>MSRIEKMSILGVRSFGIEDKDKQIITFFSPLTILVGPNGAGKTTIIECLKYICTGDFPPGTKGNTFVHDPKVAQETDVRAQIRLQFRDVNGELIAVQRSMVCTQKSKKTEFKTLEGVITRTKHGEKVSLSSKCAEIDREMISSLGVSKAVLNNVIFCHQEDSNWPLSEGKALKQKFDEIFSATRYIKALETLRQVRQTQGQKVKEYQMELKYLKQYKEKACEIRDQITSKEAQLTSSKEIVKSYENELDPLKNRLKEIEHNLSKIMKLDNEIKALDSRKKQMEKDNSELEEKMEKVFQGTDEQLNDLYHNHQRTVREKERKLVDCHRELEKLNKESRLLNQEKSELLVEQGRLQLQADRHQEHIRARDSLIQSLATQLELDGFERGPFSERQIKNFHKLVRERQEGEAKTANQLMNDFAEKETLKQKQIDEIRDKKTGLGRIIELKSEILSKKQNELKNVKYELQQLEGSSDRILELDQELIKAERELSKAEKNSNVETLKMEVISLQNEKADLDRTLRKLDQEMEQLNHHTTTRTQMEMLTKDKADKDEQIRKIKSRHSDELTSLLGYFPNKKQLEDWLHSKSKEINQTRDRLAKLNKELASSEQNKNHINNELKRKEEQLSSYEDKLFDVCGSQDFESDLDRLKEEIEKSSKQRAMLAGATAVYSQFITQLTDENQSCCPVCQRVFQTEAELQEVISDLQSKLRLAPDKLKSTESELKKKEKRRDEMLGLVPMRQSIIDLKEKEIPELRNKLQNVNRDIQRLKNDIEEQETLLGTIMPEEESAKVCLTDVTIMERFQMELKDVERKIAQQAAKLQGIDLDRTVQQVNQEKQEKQHKLDTVSSKIELNRKLIQDQQEQIQHLKSTTNELKSEKLQISTNLQRRQQLEEQTVELSTEVQSLYREIKDAKEQVSPLETTLEKFQQEKEELINKKNTSNKIAQDKLNDIKEKVKNIHGYMKDIENYIQDGKDDYKKQKETELNKVIAQLSECEKHKEKINEDMRLMRQDIDTQKIQERWLQDNLTLRKRNEELKEVEEERKQHLKEMGQMQVLQMKSEHQKLEENIDNIKRNHNLALGRQKGYEEEIIHFKKELREPQFRDAEEKYREMMIVMRTTELVNKDLDIYYKTLDQAIMKFHSMKMEEINKIIRDLWRSTYRGQDIEYIEIRSDADENVSASDKRRNYNYRVVMLKGDTALDMRGRCSAGQKVLASLIIRLALAETFCLNCGIIALDEPTTNLDRENIESLAHALVEIIKSRSQQRNFQLLVITHDEDFVELLGRSEYVEKFYRIKKNIDQCSEIVKCSVSSLGFNVH[2x];>MSTADALDDENTFKILVATDIHLGFMEKDAVRGNDTFVTLDEILRLAQENEVDFILLGGDLFHENKPSRKTLHTCLELLRKYCMGDRPVQFEILSDQSVNFGFSKFPWVNYQDGNLNISIPVFSIHGNNDDPTGADALCALDILSCAGFVNHFGRSMSVEKIDISPVLLQKGSTKIALYGLGSIPDERLYRMFVNKKVTMLRPKEDENSWFNLFVIHQNRSKHGSTNFIPEQFLDDFIDLVIWGHEHECKIAPTKNEQQLFYISQPGSSVVTSLSPGEAVKKHVGLLRIKGRKMNMHKIPLHTVRQFFMEDIVLANHPDIFNPDNPKVTQAIQSFCLEKIEEMLENAERERLGNSHQPEKPLVRLRVDYSGGFEPFSVLRFSQKFVDRVANPKDIIHFFRHREQKEKTGEEINFGKLITKPSEGTTLRVEDLVKQYFQTAEKNVQLSLLTERGMGEAVQEFVDKEEKDAIEELVKYQLEKTQRFLKERHIDALEDKIDEEVRRFRETRQKNTNEEDDEVREAMTRARALRSQSEESASAFSADDLMSIDLAEQMANDSDDSISAATNKGRGRGRGRRGGRGQNSASRGGSQRGRADTGLETSTRSRNSKTAVSASRNMSIIDAFKSTRQQPSRNVTTKNYSEVIEVDESDVEEDIFPTTSKTDQRWSSTSSSKIMSQSQVSKGVDFESSEDDDDDPFMNTSSLRRNRRSGGSLEVLFQGPDYKDDDDKGTDYKDDDDK[2x];> MWKLLPAAGPAGGEPYRLLTGVEYVVGRKNCAILIENDQSISRNHAVLTANFSVTNLSQTDEIPVLTLKDNSKYGTFVNEEKMQNGFSRTLKSGDGITFGVFGSKFRIEYEPLVACSSCLDVSGKTALNQAILQLGGFTVNNWTEECTHLVMVSVKVTIKTICALICGRPIVKPEYFTEFLKAVESKKQPPQIESFYPPLDEPSIGSKNVDLSGRQERKQIFKGKTFIFLNAKQHKKLSSAVVFGGGEARLITEENEEEHNFFLAPGTCVVDTGITNSQTLIPDCQKKWIQSIMDMLQRQGLRPIPEAEIGLAVIFMTTKNYCDPQGHPSTGLKTTTPGPSLSQGVSVDEKLMPSAPVNTTTYVADTESEQADTWDLSERPKEIKVSKMEQKFRMLSQDAPTVKESCKTSSNNNSMVSNTLAKMRIPNYQLSPTKLPSINKSKDRASQQQQTNSIRNYFQPSTKKRERDEENQEMSSCKSARIETSCSLLEQTQPATPSLWKNKEQHLSENEPVDTNSDNNLFTDTDLKSIVKNSASKSHAAEKLRSNKKREMDDVAIEDEVLEQLFKDTKPELEIDVKVQKQEEDVNVRKRPRMDIETNDTFSDEAVPESSKISQENEIGKKRELKEDSLWSAKEISNNDKLQDDSEMLPKKLLLTEFRSLVIKNSTSRNPSGINDDYGQLKNFKKFKKVTYPGAGKLPHIIGGSDLIAHHARKNTELEEWLRQEMEVQNQHAKEESLADDLFRYNPYLKRRR

The MRE11-RAD50-NBS1 (MRN) complex is a central, multifunctional factor in the detection, signaling and nucleolytic processing of DNA double-strand breaks (DSBs). The core MR complex contains two copies of both the ATPase RAD50 and the endo-/exonuclease MRE11, assembled in an elongated structure. This structure consists of a “head” module which includes MRE11 and the ATP binding cassette type nucleotide binding domains (NBDs) of RAD50, and a “tail” module formed by the coiled-coil domains (CCDs) of RAD50. Furthermore, MRN/X’s nuclease is highly regulated by trans-interacting factors that interact with a regulatory surface patch on RAD50, denoted “S site”.

The highest resolution structures were obtained by incubating MR or MH129NRN (nuclease dead mutant, hereafter referred to as ‘MRN’) with 50 bp DNA and ATP at 35 °C for 30 min, followed by addition of BeFx (producing the ATP mimic ADP•BeFx after ATP hydrolysis). Our structure resolves a single NBS1 polypeptide (651-754), which wraps around the MRE11 dimer with the highly conserved K683NFKKFKK690 motif situated across the two-fold symmetry axis. Intriguingly, the very C-terminal region of NBS1 (718-745) forms a continuous helix (“C helix”) that bridges one MRE11 catalytic domain to one RAD50NBD in the sensing state. The first part of the helix binds MRE11 via a hydrophobic interface between L719NBS1, L723NBS1, W722NBS1 and F233MRE11. The second part of the C helix is bound to the N-lobe β-sheet at the RAD50 S site. Here F744NBS1 binds into an S site pocket lined by K6RAD50, S8RAD50, I24RAD50, R83RAD50 and Q85RAD50. DNA interactions are virtually identical in MR and in MRN complexes. However, the highly positively charged C-terminus of NBS1 (K751KRRR755) binds the DNA emerging from RAD50 and induces additional DNA contacts on one side of MRN. During 3D classification, we identified two separable conformational states in MR and MRN, one with the MRE11 dimer symmetrically attached to both RAD50NBDs, and one where the MRE11 catalytic domain dimer detaches as a rigid body from one RAD50NBD. In the case of MRN, the detachment is only observed at the RAD50NBD not bound to NBS1. These observations suggest a stabilizing effect of the NBS1 C helix-S site interaction on MRN catalytic head dynamics.> MISNQQSDNGQKENIKNLGAKRARKMDTESNNGTVSDILYPECHLNSPIVKGKIAQLHTIMSLPQPYDMDDDSILVITRQKIKLNKLDKRQRSIRRLKLILTEKVNDLGKYTFIRYPEMSKEMFKLYIPGINSKVTELLLKADRTYSQMTDGLRDLWINVLSKLASKNDGSNYDLNEEINNISKVHTTYKSDKWYNPFKTWFTIKYDMRRLQKARNEITFNVGKDYNLLEDQKNFLLIHPELVLILDKQNYNGYLITPELVLMYCDVVEGRWNISACAKLDPKLQSMYQKGNNLWEVIDKLFPIMGEKTFDVISLLEPLALSLIQTHDPVKQLRGAFLNHVLSEMELIFESGESIREFLSVDYIDKILDIFNESTIDEIAEIFSFFRTFGHPPLEASIAAEKVRKYMYIEKQLKFDTVNKCHAIFCTIIINGYRERHGGQWPPVTLPDHAHEFIINAYGSNSAISYENAVDYYQSFIGIKFNKFIEPQLDEDLTIYMKDKALSPKKSNWDTVYPASNLLYRTNASNESRRLVEVFIADSKFDPHQILDYVESGDWLDDPEFNISYSLKEKEIKQEGRLFAKMTYKMRATQVLSETLLANNIGKFFQENGMVKGEIELLKRLTTISISGVPRYNEVYNNSKSHTDDLKTYNKISNLNLSSNQKSKKFEFKSTDIYNDGYETVSCFLTTDLKKYCLNWRYESTALFGETCNQIFGLNKLFNWLHPRLEGSTIYVGDPYCPPSDKEHISLEDHPDSGFYVHNPRGGIEGFCQKLWTLISISAIHLAAVRIGVRVTAMVQGDNQAIAVTTRVPNNYDYRIKKEIVYKDVVRFFDSLREVMDDLGHELKLNETIISSKMFIYSKRIYYDGRILPQALKALSRCVFWSETVIDETRSASSNLATSFAKAIENGYSPVLGYACSIFKNIQQLYIALGMNINPTITQNIKDQYFKNSNWMQYASLIPASVGGFNYMAMSRCFVRNIGDPSVAALADIKRFIKANLLDRSVLYRIMNQEPGESSFLDWASDPYSCNLPQSQNITTMIKNITARNVLQDSPNPLLSGLFTNTMIEEDEELAEFLMDRKVILPRVAHDILDNSLTGIRNAIAGMLDTTKSLIRVGINRGGLTYSLLRKISNYDLVQYETLSRTLRLIVSDKIRYEDMCSVDLAIALRQKMWIHLSGGRMISGLETPDPLELLSGVVITGSEHCKICYSSDGTNPYTWMYLPGNIKIGSAETGVSSLRVPYFGSVTDERSEAQLGYIKNLSKPAKAAIRIAMIYTWAFGNDEISWMEASQIAQTRANFTLDSLKILTPVATSTNLSHRLKDTATQMKFSSTSLIRVSRFITMSNDNMSIKEANETKDTNLIYQQIMLTGLSVFEYLFRLKETTGHNPIVMHLHIEDECCIKESFNDEHINPESTLELIRYPESNEFIYDKDPLKDVDLSKLMVIKDHSYTIDMNYWDDTDIIHAISICTAITIADTMSQLDRDNLKEIIVIANDDDINSLITEFLTLDILVFLKTFGGLLVNQFAYTLYSLKIEGRDLIWDYIMRTLRDTSHSILKVLSNALSHPKVFKRFWDCGVLNPIYGPNTASQDQIKLALSICEYALDLFMREWLNGVSLEIYICDSDMEVANDRKQAFISRHLSFVCCLAEIASFGPNLLNLTYLERLDLLKQYLELNIKEDPTLKYVQISGLLIKSFPSTVTYVRKTAIKYLRIRGISPPEVIDDWDPIEDENMLDNIVKTINDNCNKDNKGNKINNFWGLALKNYQVLKIRSITSDSDDNDRLDASTSGLTLPQGGNYLSHQLRLFGINSTSCLKALELSQILMKEVNKDKDRLFLGEGAGAMLACYDATLGPAINYYNSGLNITDVIGQRELKIFPSEVSLVGKKLGNVTQILNRVKVLFNGNPNSTWIGNMECESLIWSELNDKSIGLVHCDMEGAIGKSEETVLHEHYSVIRITYLIGDDDVVLVSKIIPTITPNWSRILYLYKLYWKDVSIISLKTSNPASTELYLISKDAYCTIMEPSEVVLSKLKRLSLLEENNLLKWIILSKKRNNEWLHHEIKEGERDYGVMRPYHMALQIFGFQINLNHLAKEFLSTPDLTNINNIIQSFQRTIKDVLFEWINITHDDKRHKLGGRYNIFPLKNKGKLRLLSRRLVLSWISLSLSTRLLTGRFPDEKFEHRAQTGYVSLADTDLESLKLLSKNIIKNYRECIGSISYWFLTKEVKILMKLIGGAKLLGIPRQYKEPEEQLLENYNQHDEFDIDDYKDDDDK;>MESDAKNYQIMDSWEEESRDKSTNISSALNIIEFILSTDPQEDLSENDTINTRTQQLSATIYQPKIKPTETSEKDSGSTDKNRQSGSSHECTTEAKDRTIDQETVQRGPGRRSSSDSRAETVVSGGISRSITNSKNGTQNTEDIDLNEIRKMDKDSIEGKVRQSADVPSEISGSDVIFTTEQSRNSDHGRSLESISTPDTRSISVVTAATPDDEEEILMKNSRTKKSSSIHQEDDKRIKKGGKGKDWFKKSKDTDNQIPTSDYRSTSKGQKKISKTTTINTDTKGQTEIQTESSGTQSSSWNLTIDNNTDRTEQTNTTPPTTTSGSTYTKESIRTNSGSKPKTQKTNGKERKDTEESNRFTERAITLLQNLGVIQSTSKLDLYQDKRVVCVANVLNNVDTASKIDFLAGLVIGVSMDNDTKLTQIQNEMLNLKADLKKMDESHRRLIENQREQLSLITSLISNLKIMTERGGKKDQNESNERVSMIKTKLKEEKIKKTRFDPLMETQGIDKNIPDLYRHAGNTLENDVQVKSEILSSYNESNATRLIPKKVSSTMRSLVAVISNSNLSQSTKQSYINELKHCKNDEEVSELMDMFNEDVNNCQHHHHHH[5x]

The RNA polymerase complex of hPIV3, like other nsNSV members, consists of the large protein (L) and a co-factor protein, the phosphoprotein (P; or VP35 in the case of the filoviruses)4. L harbors five domains including the RNA dependent RNA polymerase (RdRp) domain, polyribonucleotidyltransferase (PRNTase) domain, connector domain (CD), methyltransferase (MTase) domain and the C-terminal domain (CTD), and possesses enzymatic activities required for RNA synthesis, cap addition and cap methylation. The P protein consists of an N-terminal domain (NTD), central oligomerization domain (OD) and C-terminal X domain (XD). Here, we report the cryo-electron microscopy (cryo-EM) structures of hPIV3 L–P polymerase in monomeric and incomplete dimeric forms.

In addition to this L–P structure with one L–P copy bound with CD′ of the second copy, another main class (class 2) of particles lacking density for the second CD domain was reconstructed to a 3.3 Å resolution structure representing the monomeric L–P complex. Since these two structures show nearly the same arrangement except for the second CD domain, we used the 2.7 Å structure for further analysis.>MEEKIKELEEKVEELVKEALEKKDPAVLKKALVCVYEMKKLGMPNEKLIELLKKLVEVLKKLALERVDPAVLDLALVCVYEMKELGMPNEELIKLLKELVEVLRILALINVDPAVLDKALVCVYLMKELGMPNEELIKLLEELVEVLRILALIRVDKRVLDKAEVCIEEMEELGMPEEKIKELREELKFVREILDKIGSWLEHHHHHH[6x]

Here we describe a systematic approach to generating modular and rigid repeat protein oligomers with coincident C2 to C8 and superhelical symmetry axes that can be readily extended by repeat propagation. Repeat proteins are composed of an asymmetric structural motif that is concatenated several times in tandem within a single protein chain. From these building blocks, we demonstrate that a wide range of unbounded fibres can be systematically designed by introducing hydrophilic surface patches that force staggering of the monomers; the geometry of such fibres can be precisely tuned by varying the number of repeat units in the monomer and the placement of the hydrophilic patches. All multiplexes follow the naming convention CsHRN_Rr where s is the cyclic symmetry, HR stands for helical repeat, R is the number of repeats in a single chain and N is an index to differentiate between multiplexes of the same symmetry.

We determined the high-resolution structures of five designs from C2 to C6 symmetry by X-ray crystallography, cryogenic electron microscopy (cryoEM) or both. C6HR1_4r matches the design model with an overall r.m.s.d. of 1.97 Å. Like C5HR2_4r and many of the other two-helix repeat oligomers, the monomers of C6HR1_4r interact at the inner radius of the oligomer, but the repeats fan out towards the outer radius. The C6HR1_4r interface may be stabilized by a repetitive cation–pi interaction between tyrosine and arginine side chains of adjacent monomers. The high-resolution structure of C6HR1_4r is the widest with an outer radius of 92 Å. The inner radius is 41 Å, which is large enough to fit a C2HR dimer.>[4x]PIYDLIIKNGIICTASDIYAAEIAVNNGKVQLIAASIDP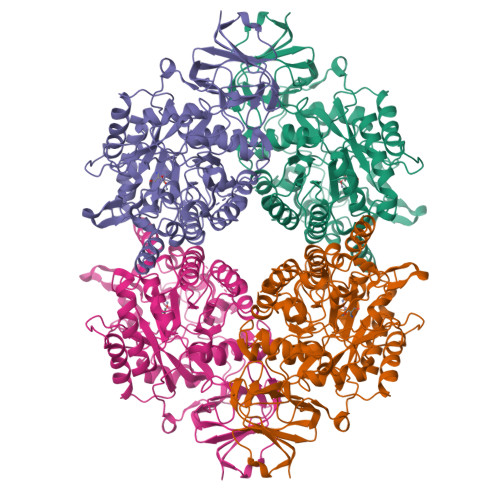SLGSEVIDAEGAFITPGGIDAHVHVDEPLKLLGDVVDTMEHATRSAVAGGTTTVVAFSTQDVSKKGPSALAESVKLDVDEYSEQTLYCDYGLHLILFQIEKPSVEARELLDVQLQAAYNDYGVSSVKMFMTYPGLQISDYDIMSAMYATRKNGFTTMLHAENGDMVKWMIEALEEQGLTDAYYHGVSRPSIVEGEATNRAITLATTMDTPILFVHVSSPQAAEVIKQAQTKGLKVYAETCPQYALLSDAITRCHHHGEVESYGVGIDLSSISESPFTNPDDRFIGSKYICSPPIRPEGTQKSIWKGMNNGTFTIVGSDHCSYNYYEKTSTASKHRAFDPENNKNGEFRYIPNGLPGVCTRMPLLYDYGYLRGNLTSMMKLVEIQCTNPAKVYGMYPQKGSILPGVSDADLVIWYPDDSKKEYNSKPKLITNKLMEHNCDYTPFEGIEIKNWPRYTIVKGKIVYKEGEILKENADGKYLKRGKSFMCTPKNEWVTEWRPKYESPGDDDDKHHHHHHHHSGD>LDNSYKMNHKRRGLCLIINNKNFDRKTGMKTRNGTDKDAENLEKTFKSLGFEVKVYNDLTAEEMQETLQEVSKEDHSDSDCFVCVLLSHGEEGLVYGTDGKIEIQELTSLFKGDKCQSLVGKPKLFFIQACRGDELDSGVEV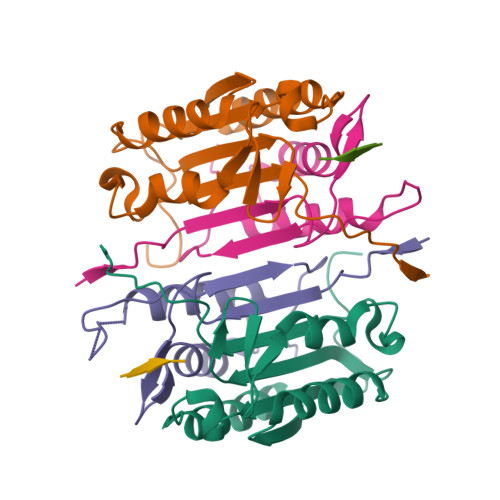[2x];>HKIPAEADFLIAYSTAPGYYSYRNTSNGSWFIQSLCEVLNKYGSELEIMEILTRVNHKVSLRSESSSNDPAFNGKKQMPCFASMLTKKLYFSP[2x];>[2x]XDEVD>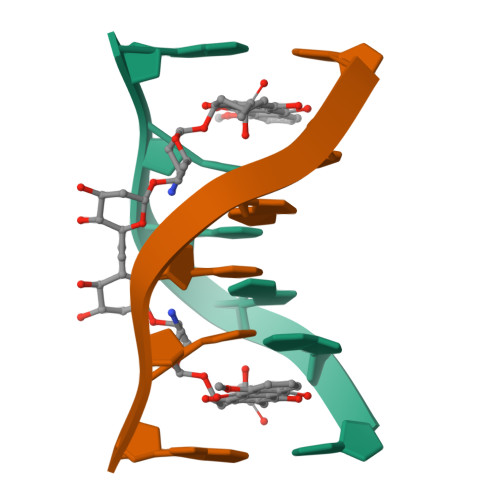 CGATCG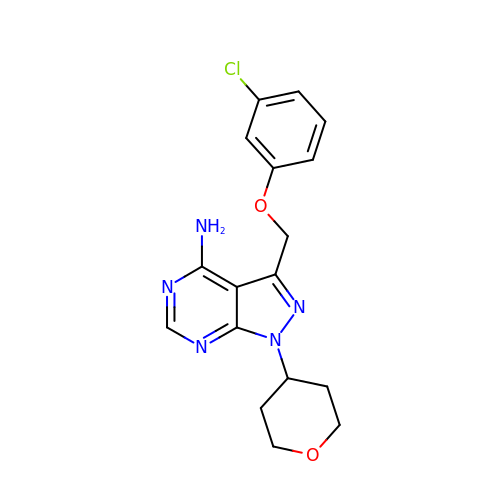3-[(3-chlorophenoxy)methyl]-1-(tetrahydro-2H-pyran-4-yl)-1H-pyrazolo[3,4-d]pyrimidin-4-amine | C17 H18 Cl N5 O2 | AUMDBEHGJRZSOO-UHFFFAOYSA-N> MATSRANDAPIVLLHGFTGWGREEMFGFKYWGGVRGDIEQWLNDNGYRTYTLAVGPLSSNWDRACEAYAQLVGGTVDYGAAHAAKHGHARFGRTYPGLLPELKRGGRIHIIAHSQGGQTARMLVSLLENGSQEEREYAKAHNVSLSPLFEGGHHFVLSVTTIATPHDGTTLVNMVDFTDRFFDLQKAVLEAAAVASNAPYTSEIYDFKLDQWGLRREPGESFDHYFERLKRSPV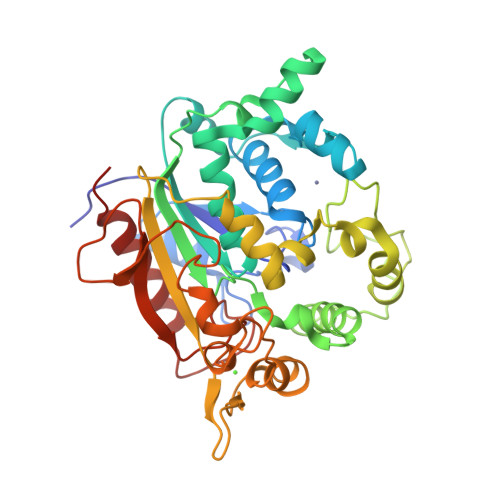WTSTDTARYDLSVPGAETLNRWVKASPNTYYLSFSTERTYRGALTGNYYPELGMNAFSAIVCAPFLGSYRNAALGIDSHWLENDGIVNTISMNGPKRGSSDRIVPYDGALKKGVWNDMGTYNVDHLEIIGVDPNPSFDIRAFYLRLAEQLASLRP> SNSITVRARGVNGQESVSLQVGGTTVQTWTLTTAMQDYTASTSLTGEIRVAFTNDATG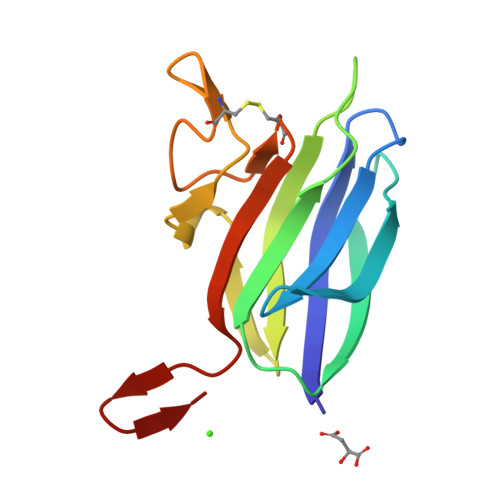RDVQVDYIVVNGQTRQAENQSVNTGVWANNQCGGSGNSEWLHCNGYISFGNVSLEHHHHHH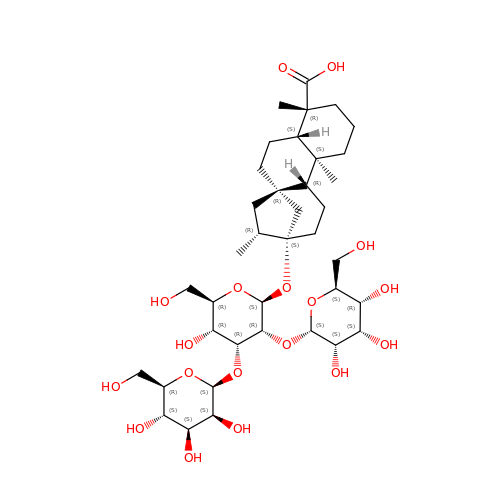(8alpha,9beta,10alpha,13alpha)-13-{[alpha-L-allopyranosyl-(1->2)-[beta-D-mannopyranosyl-(1->3)]-beta-D-allopyranosyl]oxy}kauran-18-oic acid | C38 H62 O18 | VDNFPBCVHYOBFH-LNBNFVSXSA-N>[2x]MNLDSF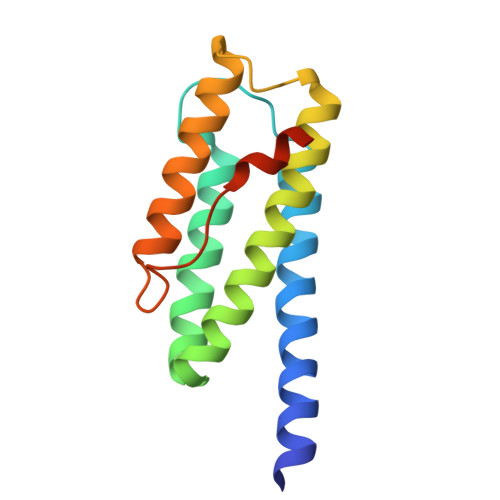KEELDDYFKEKIVKEFEKLCKELISKYEVKKPTPSPEIKKICEYLKKKHEELKDKYPEEFVKEIFKKMWEVFKKELSKQLKKLGVTNDGGEKYKIVKEDLNYLVDVIKSLEGLSDLDLNWEEIWNLEHHHHHH> MLNFKGYQIEIELKDGKRI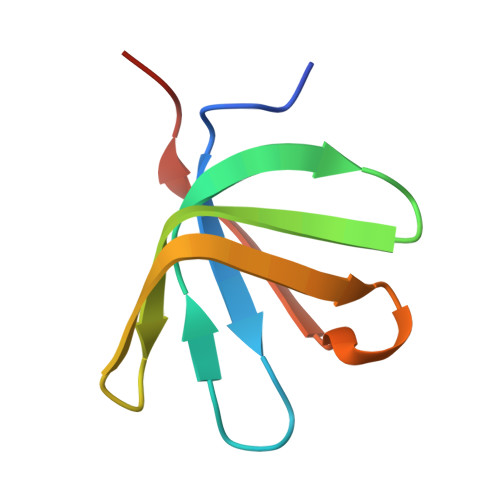TGTLKQVSPKSLTLTDAVFQDGGVSPVFKIKADKLYDLKVLKLPPNA>[3x]MHHHHHHYFSINDSKILSLQNKKNTLMDTSGYNAEVRVEGNVQLNPIFPFDFKLGSSGDDRGKVIVTQNENIVYNAMYESFSISFWIRINKWVSNLPGYTIIDSVKNNSGWSIGIISNFLVFTLKQNENSEQDINFSYDISKNAAGYNKWFFVTITTNMM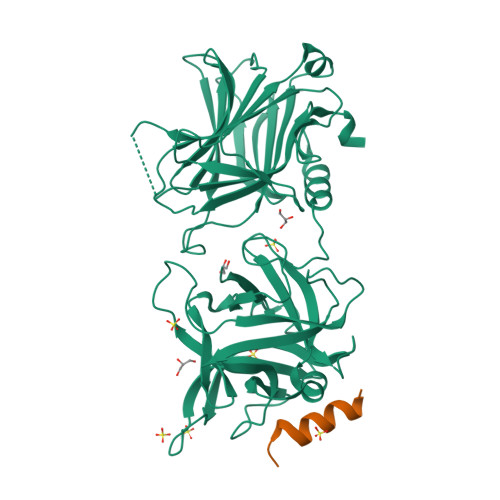GNMMIYINGKLIDTIKVKELTGINFSKTITFQMNKIPNTGLITSDSDNINMWIRDFYIFAKELDDKDINILFNSLQYTNVVKDYWGNDLRYDKEYYMINVNYMNRYMSKKGNGIVFNTRKNNNDFNEGYKIIIKRIRGNTNDTRVRGENVLYFNTTIDNKQYSLGMYKPSRNLGTDLVPLGALDQPMDEIRKYGSFIIQPCNTFDYYASQLFLSSNATTNRLGILSIGSYSFKLGDDYWFNHEYLIPVIKIEHYASLLESTSTHWVFVPAS;>[3x]GEGKEDAFSKLKEKFMNELHK> MNHKHHHHHHSSGLVPRGSAMGFDDKILLITGGTGSFGNAVMKRFLDSNIKEIRIFSRDEKKQDDIRKKYNNSKLKFYIGDVRDSQSVETAMRDVDYVFHAAALKQVPSCEFFPVEAVKTNIIGTENVLQSAIHQNVKKVICLSTDKAAYPINAMGISKAMMEKVFVAKSRNIRSEQTLICGTRYGNVMASRGSVIPLFIDKIKAGEPLTITDPDMTRFLMSLEDAVELVVHAFKHAETGDIMVQKAPSSTVGDLATALLELFEADNAIEIIGTRHGEKKAETLLTREEYAQCEDMGDYFRVPADSRDLNYSNYVETGNEKITQSYEYNSDNTHILTVEEIKEKLLTLEYVRNELNDYKASMR

The transformation of UDP-D-GlcNAc in UDP-L-FucNAc requires three enzymes (CapE, CapF and CapG) in S. aureus. The two reactions catalysed by CapE are the C-4/C-6 dehydration and the C-5 epimerization of the UDP–sugar. CapE consists of three well-defined regions: a Rossmann domain for binding the coenzyme NADPH, a substrate binding domain, and a 23-residue loop peripheral to the protein core. Herein we present the first crystal structure of CapE, revealing that this enzyme forms a stable and functional homo-hexamer.

Two structures correspond to the binary complex of the enzyme with coenzyme (wild-type protein and inactive mutein K126E). The latch is not observed in the two crystal structures of CapE with coenzyme bound because of dynamic disorder. The coenzyme engages in a dense network of non-covalent interactions with the enzyme, including polar and van der Waals forces, and hydrophobic interactions. The A–B and A–C surface areas of CapE in complex with coenzyme are significantly smaller than that of CapE with substrate analogue bound. The A–B and A–C surface areas calculated from the coordinates of CapE with coenzyme bound are reduced by 60 and 65%, respectively. The reason is the dynamic disorder occurring at these two contact regions. On the contrary, the A–F interaction surface remains essentially unchanged regardless of the ligand present in the crystal.> MAKLETVTLGNIGKDGKQTLVLNPRGVNPTNGVASLSQ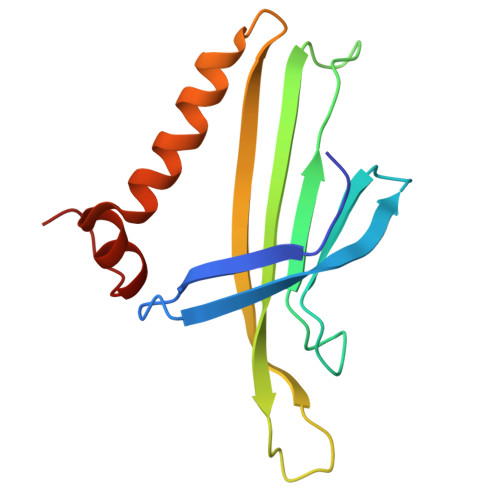AGAVPALEKRVTVSVSQPSRNRKNYKVQVKIQNPTACTANGSCDPSVTRQAYADVTFSFTQYSTDEERAFVRTELAALLASPLLIDAIDQLNPAY N~4~-[4-(4,5-dihydro-1H-imidazol-2-yl)phenyl]-N~1~-[4-(1H-imidazol-2-yl)phenyl]-2-nitrobenzene-1,4-dicarboxamide 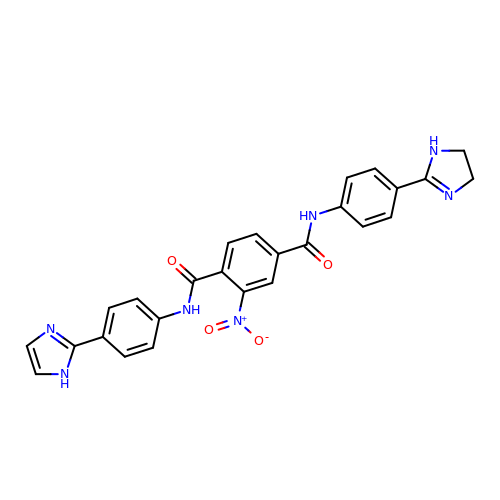| C26 H21 N7 O4 | OPTOKWNMZJTIEO-UHFFFAOYSA-N> AVDVHNLAELRIAGSTGIDAEGPDSGKHDVDLTTIVYSPPLKDNWRGFAGFG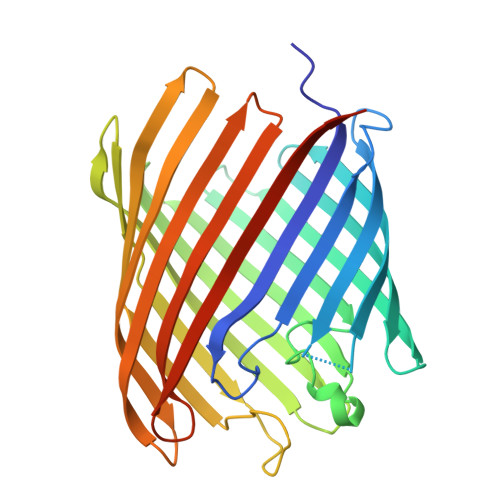YADGQFSEGKGIVRDWLAGVEWRSRNIWLEAEYAERVFNHEHKPGARLSGWYDFNDNWRIGSQLERLSHRVPLRAMKNGVTGNSAQAYVRWYQNERRKYGVSWAFTDFSDSNQRHEVSLEGQERIWSSPYLIVDFLPSLYYEQNTEHDTPYYNPIKTFDIVPAFEASHLLWRSYENSWEQIFSAGVGASWQKHYGTDVVTQLGYGQRISWNDVIDAGATLRWEKRPYDGDREHNLYVEFDMTFRFRSLEHHHHHHHHHH>AARVDQTPQTITKETGESLMFTCVLRDSNCGLSRTFWYRTKTGSTNEERISKGGRYVETVNSGSKSFSLRINDLTVEDSGTYRCRGKSWYYECPYDVYGGGTVVTVNSGQA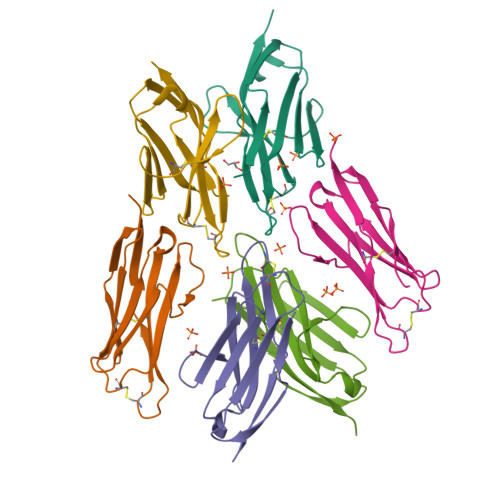GHHHHHHGDYKDDDDKG[6x]>AVRGSIIANMLQE[2x];>[2x]FTLYPYDTNYLIYTQTSDLNKEAIASYDWAENARKDEVKFQLSLAFPLWRGILGPNSVLGASYTQKSWWQLSNSEESSPFRETNYEPQLFLGFATDYRFAGWTLRDVEMGYNHDSNGRSDPTSRSWNRLYTRLMAENGNWLVEVKPWYVVGNTDDN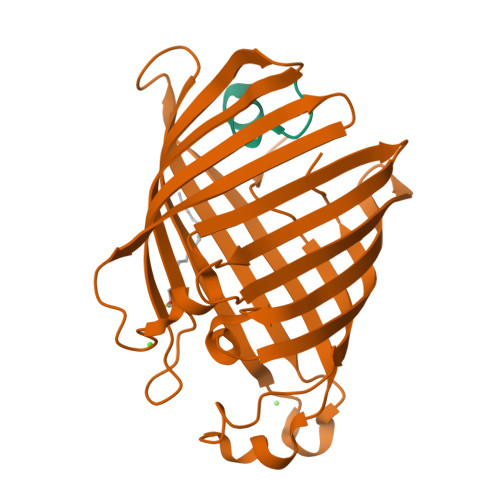PDITKYMGYYQLKIGYHLGDAVLSAKGQYNWNTGYGGAELGLSYPITKHVRLYTQVYSGYGESLIDYNFNQTRVGVGVMLNDLF In previous work, we described the inhibition of Candida albicans virulence following exposure to the 68 amino acid bacteriocin, EntV, secreted by Enterococcus faecalis. The processed, active form of EntV is 68 amino acids and is both necessary and sufficient to inhibit C. albicans biofilm formation in vitro and pathogenesis in both a nematode (Caenorhabditis elegans) infection model and a mouse model of oropharyngeal candidiasis (OPC). Notably, EntV appears to have no fungicidal or fungistatic action, but works to inhibit adhesion and hyphal morphogenesis, both of which are required for virulence in this species. The protein is further cleaved in half by the extracellular protease GelE, generating the active form of EntV which comprises the 68 amino acid C-terminus.

Unprocessed EntV136 was recombinantly purified from an E. coli strain as a selenomethionine-derivatized protein and crystallized. The structure was determined using single anomalous dispersion (SAD) phasing to 1.8 Å resolution, allowing for high resolution analysis of the structure. All residues were visible in the electron density except for the first two amino acids, the last two (169–170) and an internal region corresponding to residues 90–104; this latter region notably corresponds to the GelE cleavage site, and we postulate that there is natural flexibility in this region. The predicted disulfide bond between C106 and C167 was not observed in the structure due to the necessity of producing the protein under reducing conditions in the E. coli cytosol. However, the two cysteine residues are co-localized within 3.4 Å, consistent with the ability to form an intramolecular disulfide bond. Interestingly, the structure resembled two “clasping palms” comprised of three α-helices each. The first three helices are in the N-terminus of EntV whereas the second three are part of the C-terminus. The two palms enclose a final C-terminal helix, α7. The NTD (N-terminal domain) external face is negatively charged, while the CTD (C-terminal domain) external face is positively charged. The positive charge of the external face of the CTD is due to the presence of many lysine and arginine residues, while in contrast, the interior face that interacts with α7 is hydrophobic/neutral. α7 itself is strongly hydrophobic, as 11 of its 16 residues are hydrophobic sidechains.

> SDQLEDSEVEAVAKGLEEMYANGVTEDNFKNYVKNNFAQQEISSVEEELNVNISDASTVVQARFNWNALGSCVANKIKDEFFAMISISAIVKAAQKKAWKELAVTVLRFAKANGLKTNAIIVAGQLALWAVQCGLS N-[(5-bromo-2-methoxyphenyl)methyl]acetamide | C10 H12 Br N O2 | 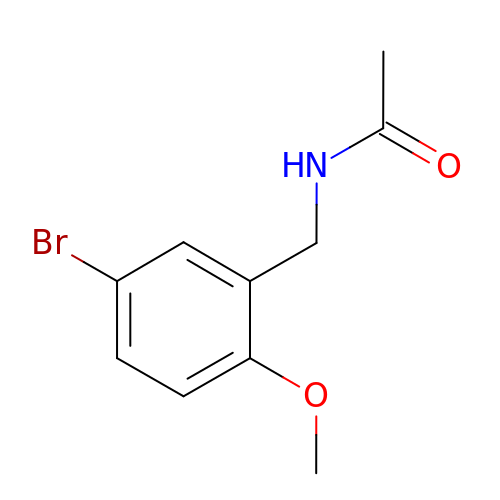XPAXEIBSVZPJBZ-UHFFFAOYSA-N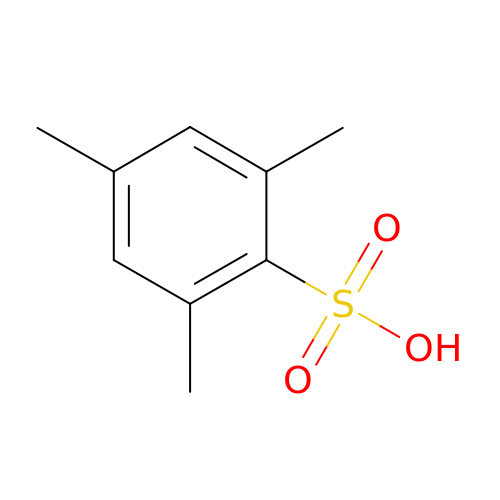2,4,6-trimethylbenzenesulfonic acid | C9 H12 O3 S | LXFQSRIDYRFTJW-UHFFFAOYSA-N> MSTKTSREIALERRKAMSDGGKKAALHSSSTKDRVRSSQDINSTGATSSNKKVLTSPSKSNIPANKIARKSTSSKLSSKELGIERRKAMSTHGKSAINSSDRTRTDVKSDIKVNKVISTEKPQALKDHNNNIKDNQVVKQNIKRRINQKRKPITNTSRDIVLARREAQSKHGKSASKQNTSAASLARRGDPDLSSREISQRVRELRSKTGSTSKQGNGKCRPCGPNKNGSKLNIADASWKVGKSETDSGQTVTGTQANRSLKTTGNEASTCRTVTGTQYMGAEVTGQFCQDKPKYKQPIRASVTTTTSGNKVTGNEVGRSEKVTGDEPGTCKNLT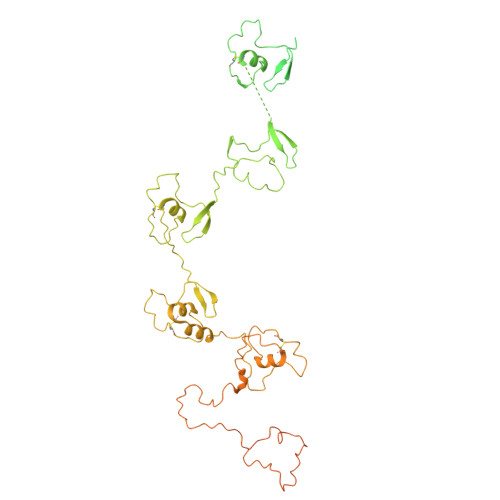GTEYISANQSKKYCGEVIKKPSKVMQSITTDGLKVSGSLPGRSSLVTGDESGSGKQLTGDQYLGSEPSPKGKSFEKVGSYDTLNGNNVTGTGVGRSDYVTGNEYGSCKNLTGDEYIGSQQYEKFCGSTPKPEARKVGLSLSSKSNLISGTMTGRSKIVTGDEPGSCKVLTGTPYAGLDQINDNCNAEIADDMKSRATVNSGNNSNARLTGLQPGIGGVMTGATKGSCKNLTGTPYIGGDQFLSNCETPPNDASYANQEKSASNSWKEFSVNSPSREKYSAKNTEGVTGNRYEDSSKITGPFDMAEDKVTGTEQFRFEPNKNMTYKQKMKQEESQNIDIPTDKKEPSKITGEGQSAGNITGDDWDRGDKVTGTEGVSARKRNPSRAGFMGAMPPVDNKRNDETEKPDFLITGSSGNTRDGQLVTFSGGARG> MDKDEAWKQVEILRRLGAKQIAYRSDDWRDLQEALKKGGDILIVDATDKDEAWKQVEILRRLGAKQIAYRSDDWRDLQEALKKGGDILIVDATDKDEAWKQVEILRRLGAKQIAYRSDDWRDLQEALKKG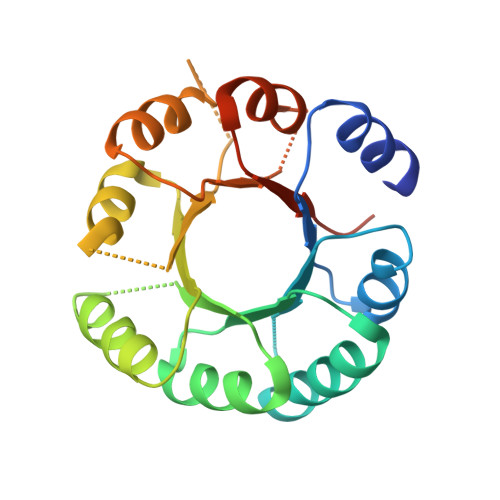GDILIVDATDKDEAWKQVEILRRLGAKQIAYRSDDWRDLQEALKKGGDILIVDATGLEHHHHHH> MTSIGTGYDLSN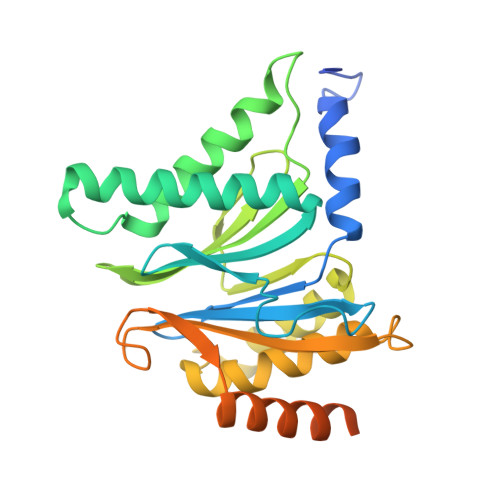SVFSPDGRNFQVEYAVKAVENGTTSIGIKCNDGVVFAVEKLITSKLLVPQKNVKIQVVDRHIGCVYSGLIPDGRHLVNRGREEAASFKKLYKTPIPIPAFADRLGQYVQAHTLYNSVRPFGVSTIFGGVDKNGAHLYMLEPSGSYWGYKGAATGKGRQSAKAELEKLVDHHPEGLSAREAVKQAAKIIYLAHEDNKEKDFELEISWCSLSETNGLHKFVKGDLLQEAIDFAQKEINGDDDEDEDDSDNVMSSDDENAPVATNANATTDQEGDIHLE> MRVLGIETSCDETGIAIYDDKKGLLANQLYSQVKLHADYGGVVPELASRDHVRKTVPLIQAALKEAGLTASDIDAVAYTAGPGLVGALLVGATVGRSLAFAWNVPAIPVHHMEGHLLAPMLEDNPPEFPFVALLVSGGHTQLISV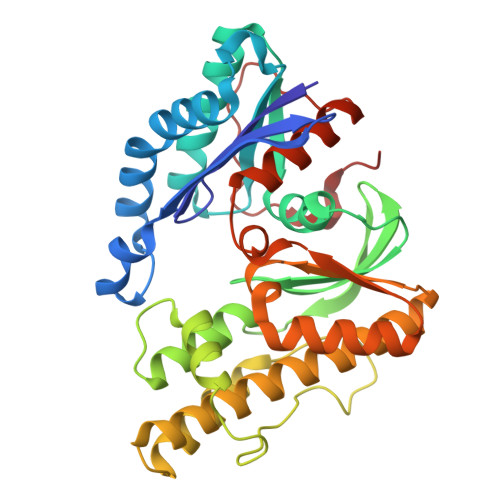TGIGQYELLGESIDDAAGEAFDKTAKLLGLDYPGGPMLSKMASQGTAGRFVFPRPMTDRPGLDFSFSGLKTFAANTIRSNGGDEQTRADIARAFEDAVVDTLMIKCKRALESTGFKRLVMAGGVSANRTLRAKLAEMMQKRRGEVFYARPEFCTDNGAMIAYAGMVRFKAGVTADLGVTVRPRWPLAELPAA>NRILPDSVDWREKGCVTEVKYQGSCGACWAFSAVGALEAQLKLKTGKLVSLSAQNLVDCSTEKYGNKGCNGGFMTTAFQYIIDNKGIDSDASYPYKAMDQKCQYDSKYRAATCSKYTELPYGREDVLKEAVANKGPVSVGVDARHPSF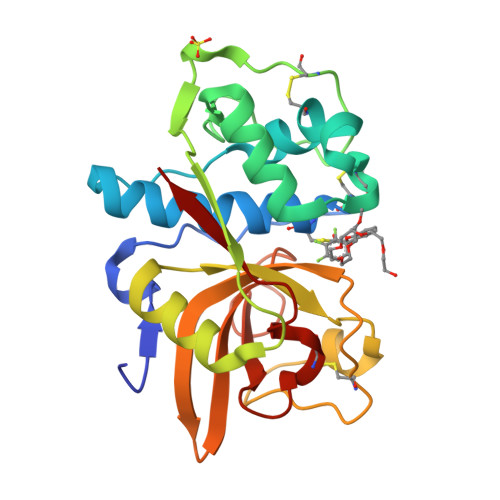FLYRSGVYYEPSCTQNVNHGVLVVGYGDLNGKEYWLVKNSWGHNFGEEGYIRMARNKGNHCGIASFPSYPEI[2x]> TFGPVFEDQPLSVLFPEESTEEQVLLACRARASPPATYRWKMNGTEMKLEPGSRHQLVGGNLVIMNPTKAQDAGVYQCLASNPVGTVVSREAILRFGFLQEFSKEERDPVKAHEGWGVMLPCNPPAHYPGLSYRWLLNEFPNFIPTDGRHFVSQTTGNLYIARTNASDLGNYSCLATSHMDFSTKSVFSKFAQLNLAAEDTRLFAPSIKARFPAETYALVGQQVTLECFAF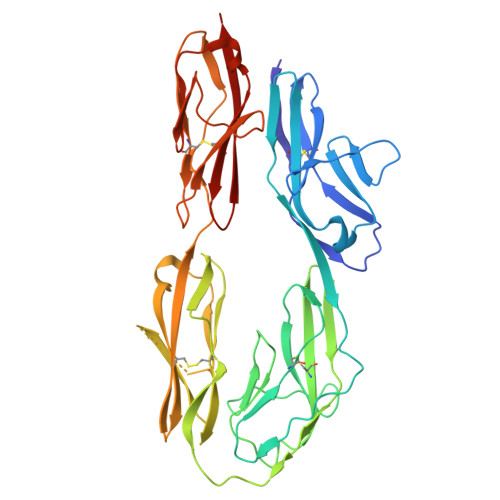GNPVPRIKWRKVDGSLSPQWTTAEPTLQIPSVSFEDEGTYECEAENSKGRDTVQGRIIVQAQPEWLKVISDTEADIGSNLRWGCAAAGKPRPTVRWLRNGEPLASQNRVEVLAGDLRFSKLSLEDSGMYQCVAENKHGTIYASAELAVQA>VTNVGEDGEPGETEPRHALSPVDMHVHTDVSFLLDRFFDVETLELSNLTGSPATHVLDPFGSTAQLAWARLLNTCTYFFSDLELSIQFKFTTTPSSVGEGFVWVKWFPVGAPTKTTDAWQLEGGGNSVRIQQLAVAGMSPTVVFKIAGSRSQACGFSVPYTSMWRVVPVFYNGWGAPTKEKATYNWLPGAHFGSILLTSDAHDKGGCYLRYRFPRANMYCPRPIPPAFTRPADKTRHKFPTNINKQ[60x];>[60x]GTTYCYSKPDGRPPSTVSDPVTRLGPTLSRHYTFKVGEWPHSQSHGHAWICPLPSDKLKKMGSFHEVVKAHHLVKNGWDVVVQVNASFAHSGALCVAAVPEYEHTHEKALKWSELEEPAYTYQQLSVFPHQLLNLRTNSSVHLVMPYIGPGPTTNLTLHNPWTIVILILSELTGPGQTVPVTMSVAPIDAMVNGPLPNPE;>[60x]APIRVVSVPESDSFMSSVPDNSTPLYPKVVVPPRQVPGRFTNFIDVAKQTYSFCSISGKPYFEVTNTSGDEPLFQMDVSLSAAELHGTYVASLSSFFAQYRGSLNFNFIFTGAAATKAKFLVAFVPPHSAAPKTRDEAMACIHAVWDVGLNSAFSFNVPYSSPADFMAVYSAEATVVNVSGWLQVYALTALTSTDIAVNSKGRVLVAVSAGPDFSLRHPVDLPDKQ

Equine rhinitis A virus (ERAV) is closely related to FMDV. The generalized picornavirus capsid is built from 60 copies of each of four structural proteins (VP1 to VP4), which are produced by cleavage of a single polyprotein by viral proteases (for a review, see reference 16). VP1 to VP3 each comprise an eight-stranded beta sandwich and form the three quasi-equivalent conformers required to build a capsid with a pseudo-T=3 surface lattice. Using cryo-electron microscopy (cryo-EM) and single particle image processing, we have determined the structure of native ERAV virions, together with the structure of a massively expanded, empty ERAV particle with large pores through the capsid layer.

The expanded structure has large pores on the particle 3-fold axes and has lost the RNA genome and the capsid protein VP4. The expanded structure thus illustrates both the limits of structural plasticity in such capsids and a plausible route by which genomic RNA might exit. The expanded capsid is much larger than the native state, with a maximum diameter (measured from the center of the particle to the tip of a pentameric turret) some 12% larger (355 Å versus 316 Å). However, the expanded state is clearly built from pentamers of the viral coat proteins, and a reasonable fit of the atomic coordinates could only be achieved as 12 isolated pentameric units. The rotation and translation of the pentameric capsomeres required to form this particle from the native state is enormous, with the points of the pentons moving by as much as ∼60 Å in three dimensions. Unsurprisingly, such large movements completely change the interacting surfaces between all adjacent pentamers, disrupting a large interface with complementary electrostatic interactions in the process. The new interface that holds the expanded particle together is obviously much smaller than in the intact particle. The core of the interaction appears to be predominantly hydrophobic in nature, with the strongest density for interpenton contacts in the expanded EM map corresponding to the location of PHE118 in VP2. The pores in the expanded capsid are the obvious route by which RNA could leave. They are located at the icosahedral 3-fold axes, and are essentially triangular, with an edge of ∼75 Å and an in-circle diameter of ∼45 Å, easily enough to allow even base-paired regions of the RNA (with a diameter of 18 to 24 Å) to leave.>[2x]SADWKAIGAYILGFAIPIILKALYMLSTRGRQTVKDNKGTRIRFKDDSSFEEVNGIRKPKHLYVSMPTAQSTMKAEEITPGRFRTIACGLFPAQVKARNIISPVMGVIGFGFFVKDWMDRIEEFLAAECPFLPKPKVASEAFMSTNK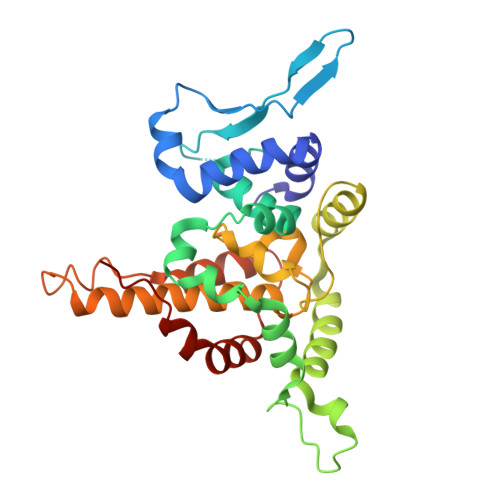MYFLNRQRQVNESKVQDIIDLIDHAETESATLFTEIATPHSVWVFACAPDRCPPTALYVAGVPELGAFFSILQDMRNTIMASKSVGTAEEKLKKKSAFYQSYLRRTQSMGIQLDQKIIILYMLSWGKEAVNHFHLGD>GSHMSKKFALTAEQRASFEKNGFIGPFDAYSPEEMKETWKRTRLRLLDRSAAAYQDLDAISGGTNIANYDRHLDDDFLASHICRPEICDRVESILGPNVLCWRTEFFPKYPGDEGTDWHQADTFANASGKPQIIWPENEEFGGTITVWTAFTDANIANGCLQFIPGTQNSMNYDETKRMTYEPDANNSVVKDG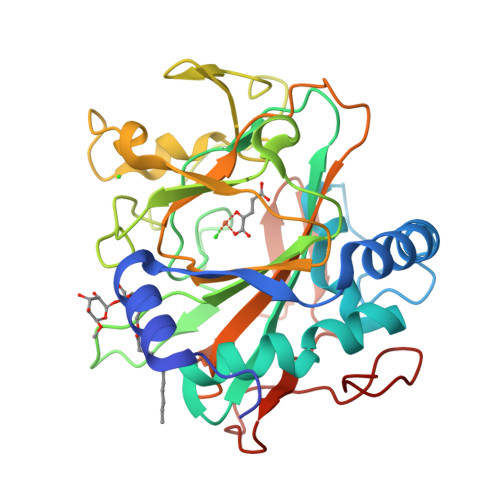VRRGFFGYDYRQLQIDENWKPDEASAVPMQMKAGQFIIFWSTLMHASYPHSGESQEMRMGFASRYVPSFVHVYPDSDHIEEYGGRISLEKYGAVQVIGDETPEYNRLVTHTTRGKKFEAV[2x]>MGGSNDFVYSIWKGPVIRAGNFALHPEVVREEVKDKRTLIGYGRFFISNPDLVDRLEKGLPLNKYDRDTFYQMSAHGYIDYPTYEEALKLGWGTSSFVKDFKPQALGDTNLFKPIKIGNNELLHRAVIPPLTRMRALHPGNIPNRDWAVEYYTQRAQRPGTMIITEGAFISPQAGGYDNAPGVWSEEQMVEWTKIFNAIHEKKSFVWVQLWVLGWAAFPDNLARDGLRYDSASDNVFMDAEQEAKAKKANNPQHSLTKDEIKQYIKEYVQAAKNSIAAGADGVEIHSANGYLLNQFLDPHSNTRTDEYGGSIENRARFTLEVVDALVEAIGHEKVGLRLSPYGVFNSMSGGAETGIVAQYAYVAGELEKRAKAGKRLAFVHLVEPR[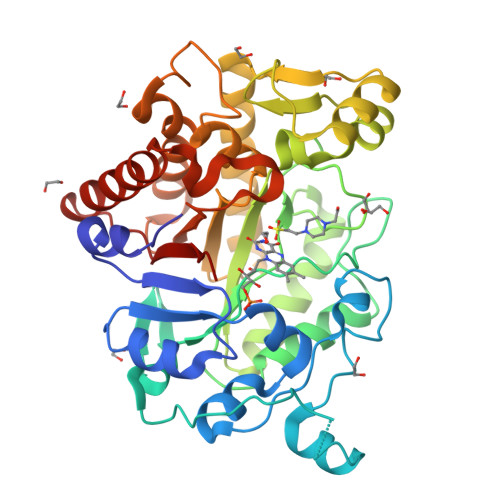2x]> MGHHHHHHMMKTKLPILGVLGGMGPVVTAEFLKSIYEYNPFIDKEQESPNVIVFSFPSAPDRTGSIDSGKEREFIDFIQVNLEHLNKLADCIVIGSCTAHYALPQIPENLKDKLISLIKIADQELQEYNEPTLLLASTGTYQKKLFQEGCTTADLIISLSESDQKLIHEMIYKVLKRGHDPLSILRDIEALLEKYNTRSYISGSTEFHLLTKSLKLKGIDSIKAIDPLSTIAQNFSQLIIKQ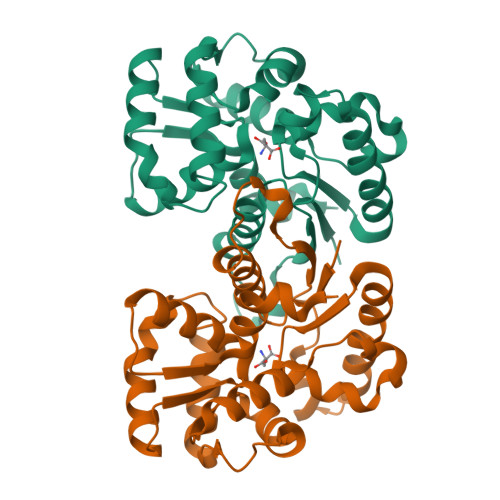AQVDLVTDCHQPSNPKSP>[4x]AMPLDAGGQNSTQMVLAPGASIFRCRQCGQTISRRDWLLPMGGDHEHVVFNPAGMIFRVWCFSLAQGLRLIGAPSGEFSWFKGYDWTIALCGQCGSHLGWHYEGGSQPQTFFGLIKDRLAEGPAD

Ito et al. showed that cereblon associates with damaged DNA binding protein 1 (DDB1) to act as a substrate receptor for the DDB1/cullin4 E3 ubiquitin ligase complex. In mammals, cereblon has a LON domain and a C-terminal thalidomide binding domain. However, homologs of the latter, also termed the CULT domain, are further found in animals and bacteria as single-domain proteins, that have all essential residues of the thalidomide binding site conserved. Architecturally, the thalidomide binding domain is a member of the β-tent fold, which consists of two antiparallel beta sheets that are oriented at an approximately right angle and pinned together at the top via a structural zinc ion.

In addition to the orthorhombic and the high-resolution trigonal crystal form, we obtained a hexagonal crystal form in a co-crystallization screen with thalidomide; we solved the structure of this third crystal form by molecular replacement, locating four monomers in the ASU. Surprisingly, only two of them are in the known thalidomide-bound conformation—the other two form an intertwined dimer and have no thalidomide bound. The two monomers of this dimer, depicted blue and pink in Fig 3, are in grossly different conformations: The blue monomer adopts an overall conformation comparable to the thalidomide-bound state but has the β3-β4 hairpin shifted in position. Therefore, the stabilizing hydrogen bond between the hairpin and the first tryptophan (W79) of the cage is broken, and the latter is found flipped out of the aromatic cage. In contrast, the conformation of the pink monomer is very different. The binding pocket is not formed and essentially all regions previously identified to be flexible are dramatically different from the thalidomide-bound conformation: In the first flexible region, the loop connecting β2 and β3 is disordered to a similar extent as in the “Wash I” structure, while the β3-β4 hairpin is shifted in position and even has another strand register. The whole second flexible region is found in an entirely different conformation—the amplitude of its largest displacement, at W79, is 30Å. Consequently, as also Y83 is not in place to anchor the second to the third region, the third flexible region is actually found in two alternative conformations, both different from the thalidomide-bound state. Intriguingly, the W79 side chain of the pink monomer reaches over to the binding site of the blue monomer to complete the aromatic cage. At the later stages of refinement, electron density of unknown origin became apparent within this cage, which was convincingly modeled as a DMSO molecule from the thalidomide stock solution.> GPLG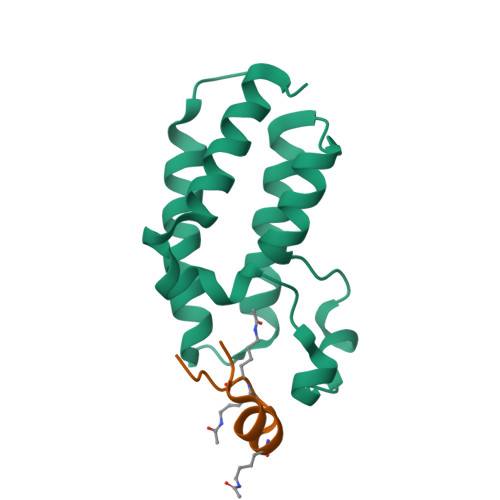SKLSEHLRYCDSILREMLSKKHAAYAWPFYKPVDAEALELHDYHDIIKHPMDLSTVKRKMDGREYPDAQGFAADVRLMFSNCYKYNPPDHEVVAMARKLQDVFEMRFAKMPDEP;> WYDVFLTRKYGKKKVAC>GSPHMTKAEKILARFNELPNYDLKAVCTGCFHDGFNEVDIEILNQLGIKIFDNIKETDKLNCIFAPKILRTEKFLKSLSFEPLKFALKPEFIIDMLKQIHSKKDKLSQININLFDYEINGINESIISKTKLPTKVFERANIRCINLVNDIPGGVDTI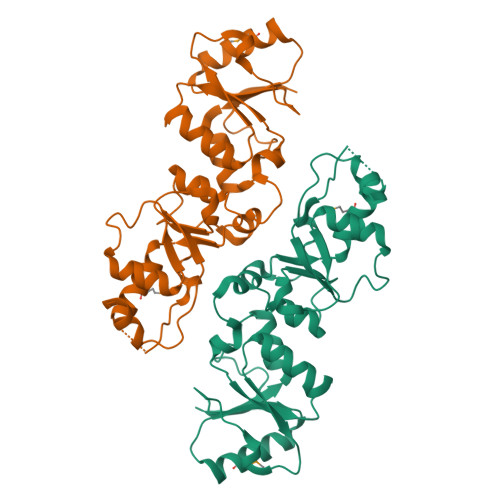GSVLKAHGIEKINVLRSKKCTFEDIIPNDVSKQENGGIFKYVLIVTKASQVKKFTKMINDRDKNETILIVEWNWCVESIFHLNVDFTSKKNVLYQKKNN[2x]> MRLLKYPLDIHNEQVNALAALGPYIILAGSGGHVMAWRQQQLVDTAFDRVMIKDLKPEVSFQVDQDTTGDIFFITGDLETLYIGSEHRLWGYSGWLCRDTNNINSVEKMNSKLLFECKSPSTITDVKYDINLGILFVLLSNENKILLFRHKTFDKLSEITIDKASKPITGIIDPTGQTFTVMTSDRSILVYQINKTGTHKLINKLTQHVQMYPLHYRISMSPQADILPVINSVKGVPNNATSCTALLDRNNNYKVTKTLVTPSSNGCRVLVYSPAFYEKPNLKKGTSTRYNLIATSGSTDGTILVWNTKRMKPLFNALQVSSTAINDMSWSQDGFTLFAISNDATLYTFAFQEKDLGVALPQTEIKSLQEVNKKLPKLEEPLAEQIPKSFPENIKLEESASAAPIPNDIGRSAVGKKPTKKKTANNQTNGIKTIQSTSMEFNTPSYTVPRDLKRKPKEATPSNIAPGSKKQKKELQPIDFLDTGLLLPNTSFSRIRLATPKIRSTFKYSPINNPNLILDVKNGSGNEQRPTIVKLTSKVLDQDQVLFQDFIPKLITICTAGDTFWSFCSEDGSIYIYSDSGRKLMAPLVLGVSISFLEACGTYLLCLTSIGELYCWNIEQKKL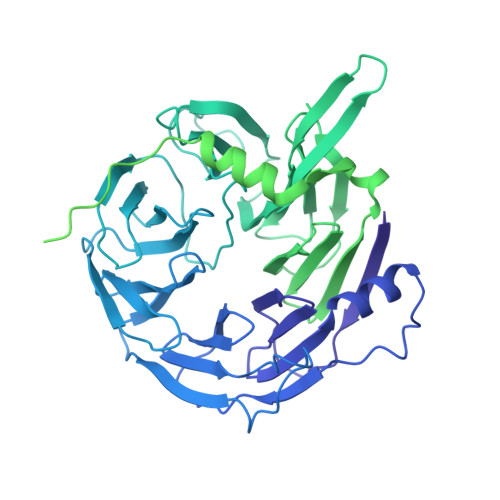AFPTNTIYPLLNPSLRYSDDILTRAENITLCSITKKGVPLVTLSNGDGYLFDKNMETWLLVSDGWWAYGSQYWDTTNTTGLSSSKANTDSFNGSESNINEIVSDIKNDNQSIINFLECKTNDELNRKGRIKNLQRFARTILMKEGFENMEEIVTLSHLENKILISIRLEEPEEFSKLMMVYCIRLSELGYMDRLNDVFQWLYDDLPISGTGSAFADKDFKRNLLKKILIACGDIRQVQRVTTRYAKEMNIIS>GPGSMQWAVGRRWAWAALLLAVAAVLTQVVWLWLGTQSFVFQREEIAQLARQYAGLDHELAFSRLIVELRRLHPGHVLPDEELQWVFVNAGGWMGAMCLLHASLSEYVLLFGTALGSRGHSGRYWAEISDTIISGTFHQWREGTTKSEVFYPGETVVHGPGEATAVEWGPNTWMVEYGRGVIPSTLAFALADTVFSTQDFLTLFYTLRSYARGLRLELT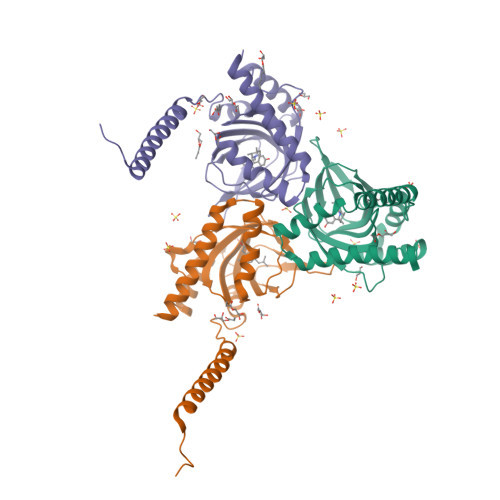TYLFGQDP[3x]On the other hand, glycogen degradation requires the glycogen debranching enzyme (GDE; GlgX), which directly catalyzes the hydrolysis of α-(1→6)-linked glucose residues and the glycogen phosphorylase (GP; GlgP) to generate glucose-1-phosphate, which feeds into primary metabolism. In this study, we identify the GDE of S. venezuelae, GlgX, as a target of c-di-GMP thus uncovering a direct link between c-di-GMP and glycogen metabolism in this bacterium. We demonstrate that c-di-GMP binding stimulates GlgX-mediated glycogen breakdown and describe crystal structures of S. venezuelae GlgX, which reveal the molecular mechanism by which c-di-GMP activates GlgX. GlgX is a 79 kDa protein that contains a putative carbohydrate-binding module (CBM_48; PF02922) and alpha amylase, catalytic domain (PF00128).

To elucidate the molecular mechanism of c-di-GMP binding by GlgX we crystallized the S. venezuelae GlgX-c-di-GMP complex and solved the structure to 3.34 Å resolution. Strikingly, in the structure, a c-di-GMP monomer is bound at each end of an antiparallel GlgX dimer. The c-di-GMP molecules, bound at each end of the GlgX molecule, make contacts to GlgX residues 31–51 from the N-domain of one GlgX subunit and residues 430–437 and 628–638 from the Central and C-domain of the other GlgX subunit. Residues in the GlgX N-domain provide most of the base specifying contacts with the c-di-GMP. In particular, the N1 and N2 atoms of one guanine base are contacted by the side chain of Glu47 while the side chain of Arg56 makes a hydrogen bond with the O6 atom of the guanine. Cation-π interactions to this guanine base are provided by Arg31 and Arg49. There are also two hydrogen bonds from residues in the Central domain of the other subunit to this guanine base; the main chain amide nitrogen of Gly436 hydrogen bonds to the guanine N2, while the side chain of Arg438 hydrogen bonds with the O6 atom of the guanine and also stacks with the guanine base along with the side chain of Arg579. The two c-di-GMP phosphates are contacted from the side chains of Ser629 and Gln433. Specifically, c-di-GMP binding leads to a restructuring of two loops formed by residues 432–442 and 579–593 within the C-domain region bound by the second messenger. Thus, these analyses indicate that c-di-GMP binding acts as an allosteric regulator of GlgX to stabilize its active state.

>[4x]GSHMQVWPGQAYPLGATYDGAGTNFAVFSEAAHRIELCLLHDDGSETAVELRETDAFVRHAYLPGVMPGQRYGFRVHGPYAPERGLRCNAAKLLLDPYARAVSGRVRWGEAVYGYPFGRPDARNDLDSAPDTMTSVVVNPYFDWGDDRRPRTEYHHTVIYEAHVKGLTMLHPDLPEELRGTYAGLAHPSVIGHLRELGVTALELMPVHQFVNDHRLVDAGLSNYWGYNTIGFFAPHNAYASWGDRGQQVLEFKSAVRALHQAGIEVILDVVYNHTAEGNHLGPTLSMRGLDNPSYYRLADDPRYYMDTTGTGNSLLMRSPHVLQLIMDSLRYWVTEMHVDGFRFDLAATLARQFHEVDRLSSFFDLVQQDPVVSQVKLIAEPWDVGEGGYQVGNFPPLWTEWNGKYRDCVRDLWRGEPRTLAEFASRLTGSSDLYQDDGRRPLASVNFVTCHDGFTLRDLVSYNEKRNEANGEGNRDGENYNRSWNCGEEGETEDVGITELRARQMRNFLATLMLSQGVPMLSHGDEFGRTQGGNNNAYCQDNEVSWVRWPKENSEAEATLLRFTRSMVRLRREHPVFRRRRFFHGRPVEGTHDELTDIAWFTPEGEEMTSRDWQAAHAQALTVFLNGNAISEPGTQGERIADDSFLLMFNASAKELEFVVPDSHGRYWRMVVDTSDPEGMPPQQGPELAGGERVTLAPLSLTVLRRPA>[4x]MSN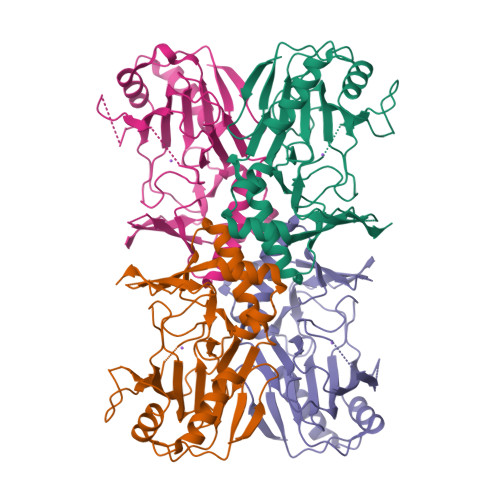AALATAPHALELDVHPVAGRIGAEIRGVKLSPDLDAATVEAIQAALVRHKVIFFRGQTHLDDQSQEGFAKLLGEPVAHPTVPVVDGTRYLLQLDGAQGQRANSWHTDVTFVEAYPKASILRSVVAPASGGDTVWANTAAAYQELPEPLRELADKLWAVHSNEYDYASLKPDIDPAKLERHRKVFTSTVYETEHPVVRVHPISGERALQLGHFVKRIKGYSLADSQHLFAVLQGHVTRLENTVRWRWEAGDVAIWDNRATQHYAVDDYGTQPRIVRRVTLAGEVPVGVDGQLSRTTRKG>SNATGFLVSFMVDARGGSMRGSRHNGLRVVIPPRTCAAPTRITCRLVKPQKLSTPPPLAEEEGLASRIIALGPTGAQFLSPVIVEIPHFASHGRGDRELVVLRSENGSVWKEHRSRYGESYLDQILNGMDEE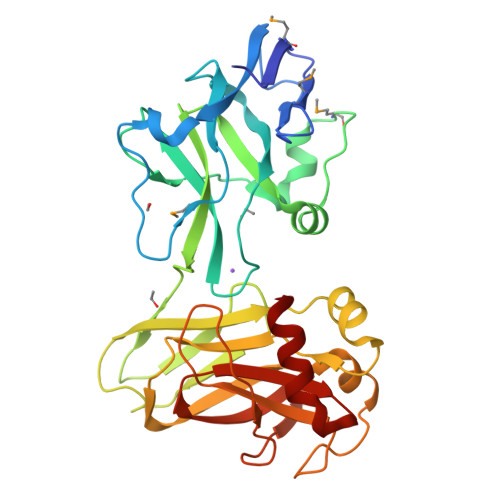LGSLEELEKKRVCRIITTDFPLYFVIMSRLCQDYDIIGPEGGSLKSKLVPLVQATFPENAVTKRVKLALQAQPVPDELVTKLLGNQATFSPIVTVEPRRRKFHRPIGLRIPLPPSWTDNPRDSGEGDTTSLRLLCSVIGGTDQAQWEDITGTTKLVYANECANFTTNVSARFWLSDCPRTAEAVNFATLLYKEL[3x]> STSKDHVKSQIPRLSAINDLHKIWPTVEEHGAAIIESFLSLDIVRRL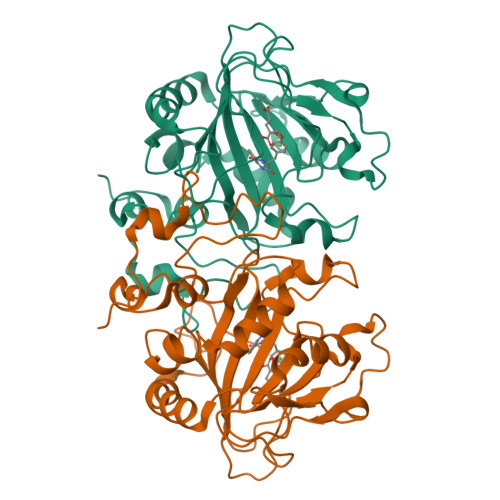NEEVDPFVKIEPIPAAKTKDHPNHILSTTTRLVNVLAPISKAYREDVLNSKVLHRICSDAFHVYGDYWVLMGAVMELAPSNPAQPLHRDMRFSHPIVEYLKPDAPATSINFLVALSPFTAENGATHVILGSHKWQNLSNVSMDATVRALMNPGDALLITDSTIHCGGAETTGTETRRLLTITMGISQLTPLESNLAVPRPVIESLTPLAQRLLGWASQRSAAPRDIGLLTIRGNSIEKTMNLKAEQPLHDDEAEPLCRETIA>MGSELETAMETLINVFHAHSGKEGDKYKLSKKELKELLQTELSGFLDAQKDVDAVDKVMKELDENGDGEVDF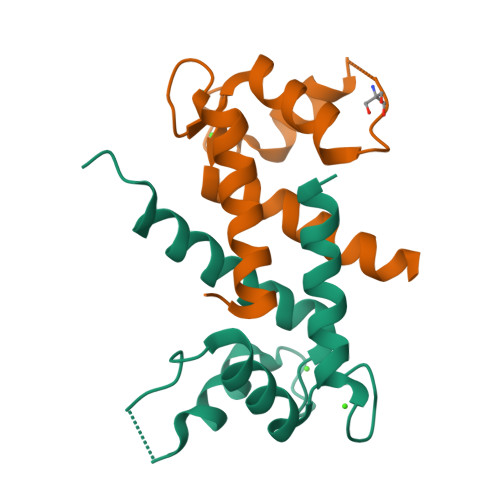QEYVVLVAALTVACNNFFWENS[3x]> GDQVEQSPSALSLHEGTDSALRCNF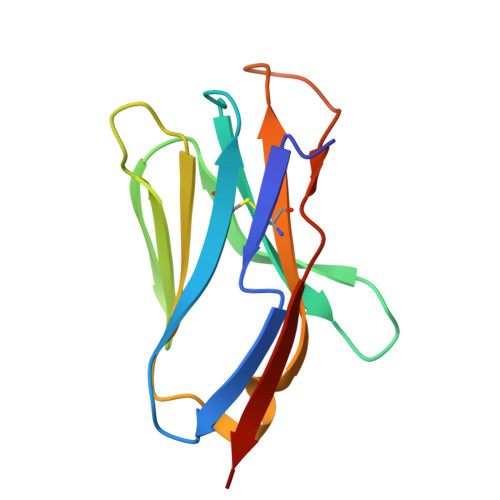TTTMRSVQWFRQNSRGSLISLFYLASGTKENGRLKSAFDSKERRYSTLHIRDAQLEDSGTYFCAAEASSGAWQLIFGSGTQLTVMPVT> GDRVADVIESSIGDSVSRALTQALPAPTGQNTQVSSHRLDTGEVPALQAAEIGASSNTSDESMIETRCVLNSHSTAETTLDSFFSRAGLVGEIDLPLEGTTNPNGYANWDIDITGYAQMRRKVELFTYMRFDAEFTFVACTPTGQVVPQLLQYMFVPPGAPKPESRE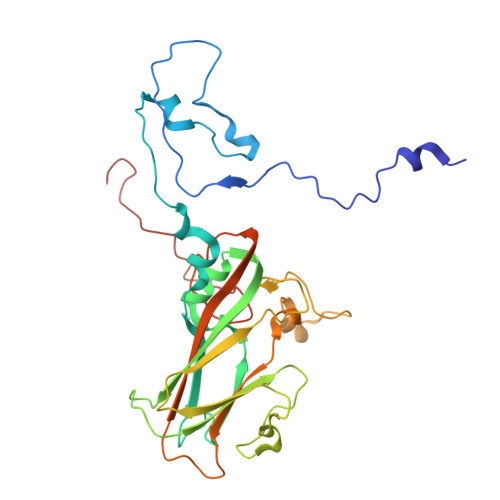SLAWQTATNPSVFVKLTDPPAQVSVPFMSPASAYQWFYDGYPTFGEHKQEKDLEYGACPNNMMGTFSVRNVGSSKSKYPLVVRIYMRMKHVRAWIPRPMRNQNYLFKANPNYAGNSIKPTGTSRTAITTLG Monkeypox is a disease with pandemic potential. It is caused by the monkeypox virus (MPXV), a double-stranded DNA virus from the Poxviridae family, that replicates in the cytoplasm and must encode for its own RNA processing machinery including the capping machinery. Here, we present crystal structures of its 2′-O-RNA methyltransferase (MTase) VP39 in complex with the pan-MTase inhibitor sinefungin and a series of inhibitors that were discovered based on it. The structure revealed a mixed α/β fold that resembles the Rossmann fold. The catalytic tetrad (Lys41, Asp138, Lys175, Glu218 for MPXV) is absolutely conserved among these unrelated viruses including the conformation of these residues.

We identified several compounds that inhibited the VP39 MTase significantly better than sinefungin. Among them, three (TO1111, TO1116, TO1119) had a relatively small substituent (small aliphatic chain or iodine atom) and five (TO427, TO494, TO500, TO504, TO507) had a large aromatic or heterocyclic substituent. Surprisingly, the efficacy of these compounds was very similar (IC50 = 0.08−0.17 µM) and an order of magnitude better than sinefungin (IC50 = 2.3 µM). To confirm our hypothesis that the inhibitors use the discovered water-filled cavity we performed a crystallographic analysis. We used the same approach as with sinefungin and we were able to obtain well diffracting crystals for five compounds (TO427, TO494, TO500, TO507, TO1119). In each case the electron density for the inhibitor was well visible allowing us to unambiguously model the inhibitor although the electron density for the large 7-deaza substituents was less defined than that for the SAH scaffold of the molecule. The crystallographic analysis revealed that in each case the moiety attached to the 7-deaza position is located within the water cavity. In the case of TO1119 that bears the large iodine atom at the 7-deaza position of the nucleobase only the water molecules near the iodine bound to the 7-deaza position were rearranged. TO1119 that only slightly disrupts the water network has IC50 = 128 nM while all the inhibitors with bulky substituents had a lower IC50 except for the only substituent that is able to form a hydrogen bond, the TO500 that possesses a benzimidazole heterocycle. These results suggest that for optimal inhibitor binding it is probably important to disrupt the water network, but it is not important to replace it with other hydrogen bonds.

>[2x]MDVVSLDKPFMYFEEIDNELDYEPESANEVAKKLPYQGQLKLLLGELFFLSKLQRHGILDGATVVYIGSAPGTHIRYLRDHFYNLGVIIKWMLIDGRHHDPILNGLRDVTLVTRFVDEEYLRSIKKQLHPSKIILISDVRSKRGGNEPSTADLLSNYALQNVMISILNPVASSLKWRCPFPDQWIKDFYIPHGNKMLQPFAPSYSAEMRLLSIYTGENMRLTRVTKSDAVNYEKKMYYLNKIVRNKVVINFDYPNQEYDYFHMYFMLRTVYCNKTFPTTKAKILFLQQSIFRFLNIPTTSTEKVSHE>[2x]MGHHHHHHVEKVATNVNLKDQFWKRYIDVVRHEVIPYQWEALNDRIPDAEPSHAIENFRIAAGESDGEFYGMVFQDSDVAKWLEAVAYLLETKRDPELEKLADDVIELLGRAQQPDGYLNTYYTIKEPGKRWMNLRDNHELYCAGHLIEAAVAYFRATGKRRFLDIMCKYADYIGTVFGRGEGQIPGYDGHQEIELALLKLYEVTGNENYLKLSQYFIDQRGQQPYYFDQEKEARGETEPFWYDGGYRYHQAHIPVREQKQAVGHAVRALYMYT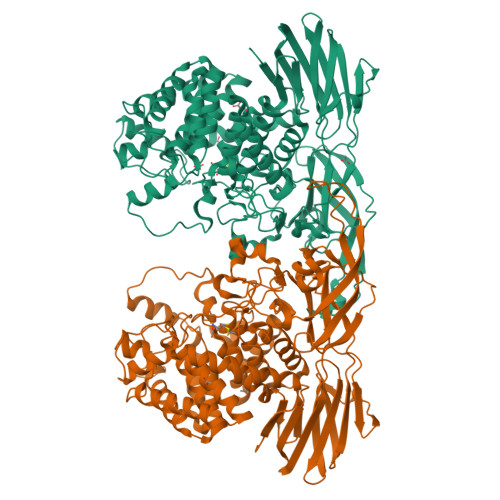AMAGLAAKMGDESLKQACQTLWENVTKRQMYITGGVGSSAFGESFTFDFDLPNDTAYAETCASIALVFWTRRMLELEMDGKYADVMERALYNGTISGMDLDGKKFFYVNPLEVWPKACERHDKRHVKPVRQKWFSCACCPPNLARLIASIGHYIYLQTSDALFVHLYVGSDIQTEIDGRSVKIMQETNYPWDGTVRLTVSPESAGEFTLGLRIPGWCRGAEVTINGEKVDIVPLIKKGYAYIRRVWQQGDEVKLYFPMPVERIKAHPQVRANAGKVALQRGPIVYCLEEVDNGPNLANLFLPRDAKLEAHFEPDLLEGVVVITGIAERVDESAWNDELYRPIEPRTYKVPFRAIPYYAWCNRGEGEMVVWVNEK> PLGSKLLLMGRSGSGKSSMRSIIFSNYSAFDTRRLGATIDVEHSHLRFLGNMTLNLWDCGGQDVFMENYFTKQKDHIFQMVQVLIHVFDVESTEVLKDIEIFAKALKQLRKYSPDAKIFVLLHKMDLVQLDKREELFQIMMKNLSETSSEFGFPNLIGFPTSIWDESLYKAWSQIVCSLIPNMSNHQSNLKKFKEIMNALEIILFERTTFLVICSSNGENSNENHDSSDNNNVLLDPKRFEKISNIMKNFKQSCTKLKSGFK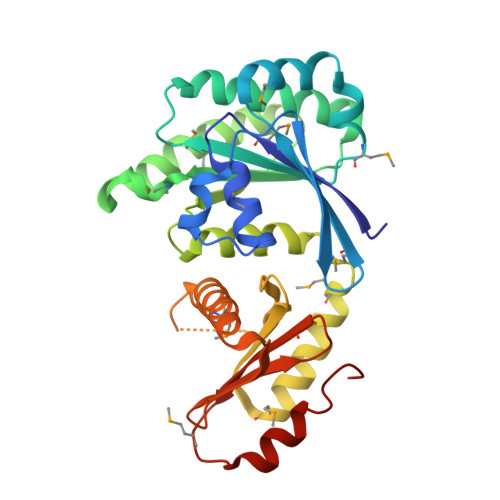TLILNNNIYVSELSSNMVCFIVLKDMNIPQELVLENIKKAKEFFQ>MKFLTTN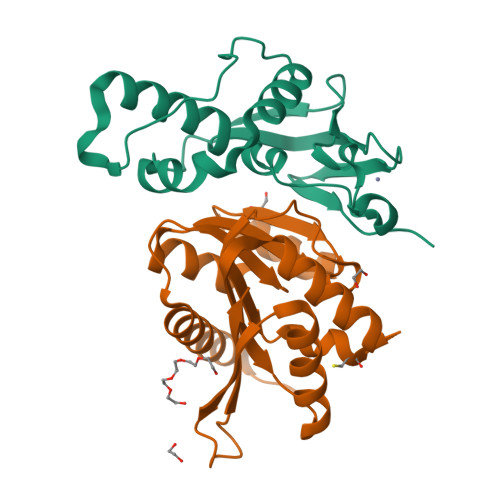FLKCSVKACDTSNDNFPLQYDGSKCQLVQDESIEFNPEFLLNIVDRVDWPAVLTVAAELGNNALPPTKPSFPSSIQELTDDDMAILNDLHTLLLQTSIAEGEMKCRNCGHIYYIKNGIPNLLLPPHLV[2x];>[2x]MSRPEELAPPEIFYNDSEAHKYTGSTRVQHIQAKMTLRALELLNLQPCSFILDIGCGSGLSGEILTQEGDHVWCGLDISPSMLATGLSRELEGDLMLQDMGTGIPFRAGSFDAAISISAIQWLCNADTSYNDPKQRLMRFFNTLYAALKKGGKFVAQFYPKNDDQVDDILQSAKVAGFSGGLVVDDPESKKNKKYYLVLSSGHHHHHH> AMNLIFLGTSAGVPTRTRNVTAILLNLQHPTQSGLWLFDCGEGTQHQLLHTAFNPGKLDKIFISHLHGDHLFGLPGLLCSRSMSGIIQPLTIYGPQGIREFVETALRISGSWTDYPLEIVEIGAGEILDDGLRKVTAYPLEHPLECYGYRIEEHDAPGALNAQ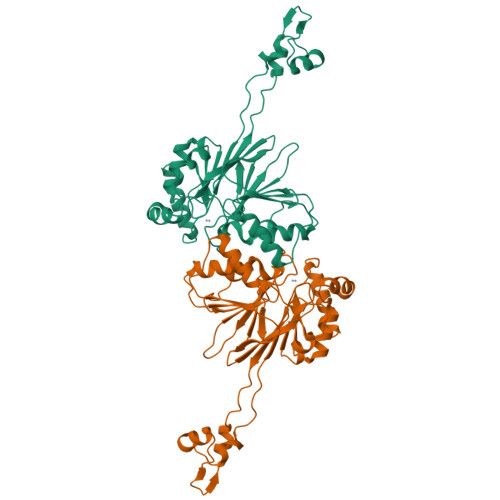ALKAAGVPPGPLFQELKAGKTITLEDGRQINGADYLAAPVPGKALAIFGDTGPCDAALDLAKGVDVMVHEATLDITMEAKANSRGHSSTRQAATLAREAGVGKLIITHVSSRYDDKGCQHLLRECRSIFPATELANDFTVFNV>MPCTEQITLYTTTFSPYGHRAHIALEEAGAEYTLCQINVHRDKPEWYKRVNPLGKVPAITFGGPQVPPDEPSPESEKLVESLALLEFVADVFPEAKLLPASPVQRARARAFIAIYQNYLHDQFRDAF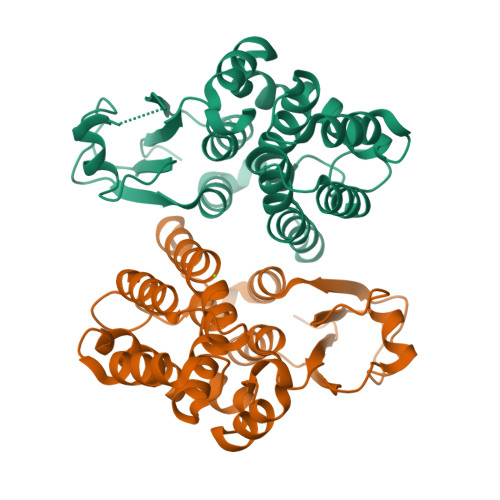FRGEPVGPFLQALETLQSALPPAGFAVGEWSLAEAAVAPFLARMMLYLDAGLGKYSEADGETMRAALASERFARISQYVRDIRARASFVKSWGGDDVQLEAAKAIPMLRRPAHHHHHH[2x]>[2x]ASMKWFRFEQDGRARIGVEEAGHRYDVTPQVYTDSLLEVIVRGFEMDVDLDVAPRLTDHVRLLAPYLPPRNVICVGKNYADHIKEMDTAGAGKFVLFTKAPSSIVGPFDPIERHADLT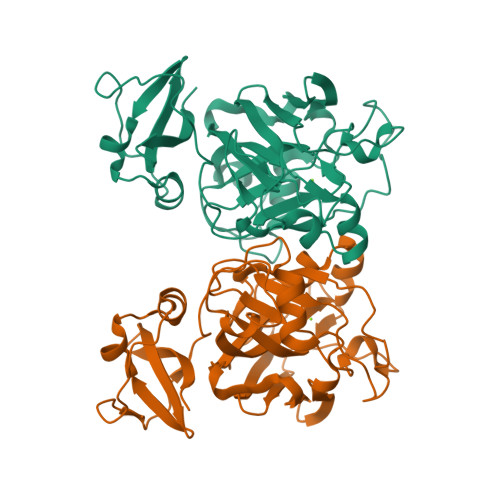QQLDYEGELAIIIGTTGRDLTPENALEHVFGYSIINDVTARDLQKEHVQFFRGKSLDGFCPFGPVIVTEDAFDPADVLVETRVNGELRQSGSTKLMLRDVVTILTEVSRGMTLEAGDVIATGTPAGVGHGMKPPVYLQDGDVIDVSIEGIGHLQNQVKARRHHHHHH>MSDAAPSLSNLFYDPTYNPGQSTINYTSIYGNGSTITFDELQGLVNSTVTQAIMFGVRCGAAALTLIVMWMTSRSRKTPIFIINQVSLFLIILHSALYFKYLLSNYSSVTYALTGFPQFISRGDVHVYGATNIIQVLLVASIETSLVFQIKVIFTGDNFKRIGLMLTSISFTLGIATVTMYFVSAVKGMIVTYNDVSATQDKYFNASTILLASSINFMSFVLVVKLILAIRSRRFLGLKQFDSFHILLIMSCQSLLVPSIIFILAYSLKPNQGTDVLTTVATLLAVLSLPLSSMWATAANNASKTNTITSDFTTSTDRFYPGTLSSFQTDSINNDAKSSLRSRLYDLYPRRKETTSDKHSERTFVSETADDIEKNQFYQLPTPTSSKNTRIGPFADASYKEGEVEPVDMYTPDTAADEEARKFWTEDNNNL[2x];>TVSTQTIGDESDPFLQNKRANDVIEQSLQLEKQRDKNEIKLLLLGADNSGKSTVLKQLKLLHGGSGGSGGTTGITETEFNIGSSKFKVLDAGGQRSERKKWIHCFEGITAVLFVLDMSDYNRMHESIMLFDTLLNSKWFKDTPFILFLNKIDLFEEKVKSMPIRKYFPDYQGRVGDAEAGLKYFEKIFLSLNKTNKPIYVKRTCATDTQTAKFILSAVTDLIIQQNLKKIGII[2x];> MAAHQMDSITYSNNVTQQYIQPQSLQDISAVEDEIQNKIEAARQESKQLHAQINKAKHKIQDASLFQMANKVTSLTKNKINLKPNIVLKGHNNKISDFRWSRDSKRILSASQDGFMLIWDSASGLKQNAIPLDSQWVLSCAISPSSTLVASAGLNNNCTIYRVSKENRVAQNVASIFKGHTCYISDIEFTDNAHI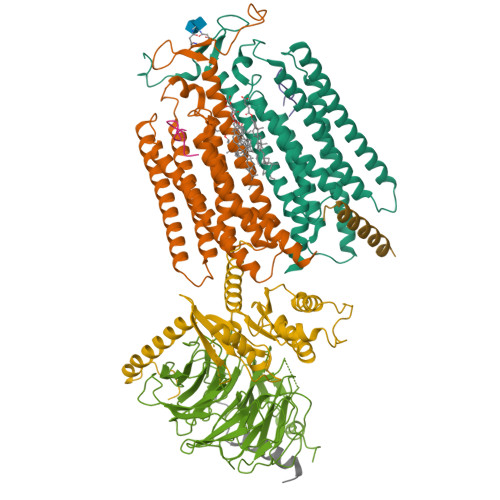LTASGDMTCALWDIPKAKRVREYSDHLGDVLALAIPEEPNSENSSNTFASCGSDGYTYIWDSRSPSAVQSFYVNDSDINALRFFKDGMSIVAGSDNGAINMYDLRSDCSIATFSLFRGYEERTPTPTYMAANMEYNTAQSPQTLKSTSSSYLDNQGVVSLDFSASGRLMYSCYTDIGCVVWDVLKGEIVGKLEGHGGRVTGVRSSPDGLAVCTGSWDSTMKIWSPGYQ;> TSVQNSPRLQQPQEQQQQQQQLSLKIKQLKLKRINELNNKLRKELSRERITASNACLTIINYTSNTKDYTLPELWGYPVAGSNHFIEGLKNAQKNSQMSNSNSVSSTLM;>[2x]WHWLQLKPGQPMY> QASARPSSSMADFRKFFAKAKHIVIISGAGVSAESGVPTFRGAGGYWRKWQAQDLATPLAFAHNPSRVWEFYHYRRE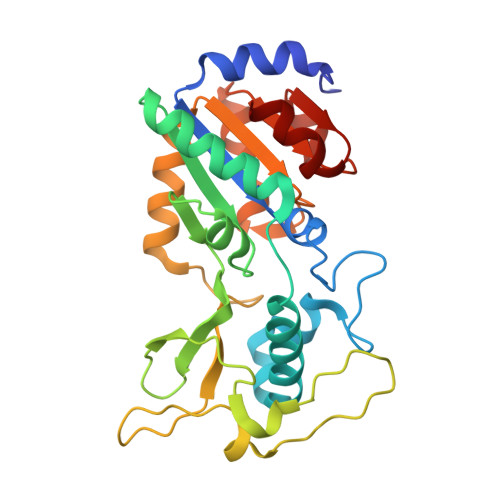VMGSKEPNAGHRAIAECETRLGKQGRRVVVITQNIDELHRKAGTKNLLEIHGSLFKTRCTSCGVVAENYKSPICPALSGKGAPEPGTQDASIPVEKLPRCEEAGCGGLLRPHVVWFGENLDPAILEEVDRELAHCDLCLVVGTSSVVYPAAMFAPQVAARGVPVAEFNTETTPATNRFRFHFQGPCGTTLPEALA> VTSL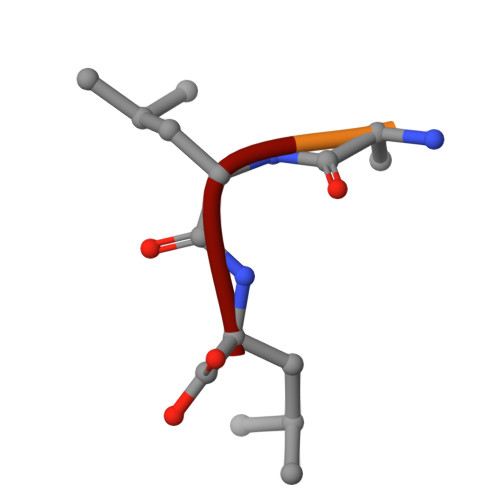L>MAIAHLATEYVFSDFLLKEPTEPKFKGLRLELAVDKMVTCIAVGLPLLLISLAFAQEISIGTQISCFSPSSFSWAQAAFVDSYCWAAVQQKSSLQSESGNLPLWLHKFFPYILLLFAILLYLPALFWRFSAAPHLCSDLKFIMEELDKVYNRAIKAAKSARDLDLRDGPGPPGVTENVGQSLWEISESHFKYPIVEQYLKTKKNSSHLIMKYISCRLVTFVVILLACIYLSYYFSLSSLSDEFLCSIKSGVLKNDSTIPDRFQCKLIAVGIFQLLSLINLIVYALLIPVVVYTFFIPFRQKTDILKVYEILPTFDVLHFKSEGYNDL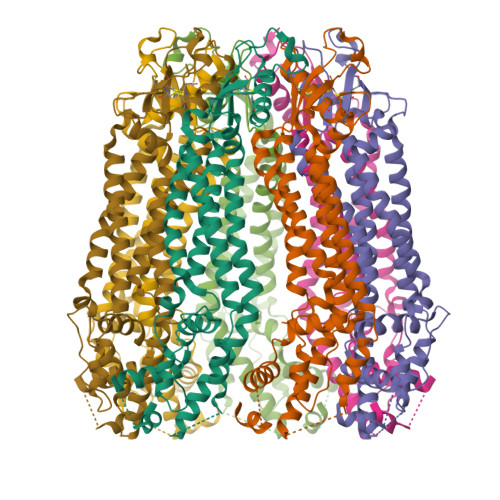SLYNLFLEENISELKSYKCLKVLENIKSNGQGIDPMLLLTNLGMIKMDIIDGKIPTSLQTKGEDQGSQRVEFKDLDLSSEAAANNGEKNSRQRLLNPSCGSAAAENLYFQGHHHHHH[7x]> GS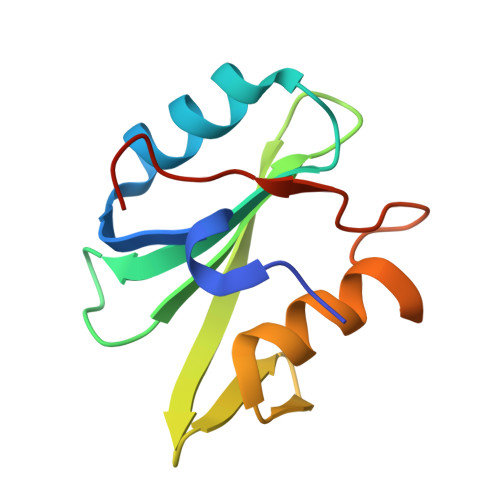TAPPTNQWYHGKLDRTIAEERLRQAGKSGSYLIRESDRRPGSFVLSFLSQMNVVNHFRIIAMSGDYYIGGRRFSSLSDLIGYYSHVSSLLKGEKLLYPVAPPEPVED> PDQFRAIIESPEGAGHVGYQYRRNTGSTMRMVSDVLDERVSLWDFHCDPSGNVIQPGPNVDSRQYLQAAIDYVSSNGGGTITIPAGYTWYLGSYGVGGIAGHSGIIQLRSNVNLNIEGRIHLSPFFDLKPFQVFVGFDNGDPASSGNLENCHIYGHGVVDFGGYEFGASSQLRNGVAFGRSYNCSVTGITFQNGDVTWAITLGWNGYGSNCYVRKCRFINLVNSSVNANHSTVYVNCPYSGVESCYFSMSSSFARNIACSVALHQHDTFYRGSTVNGYCRGAYVVMHAAEAAGAGSYAYNMQVENNIAVIYGQFVILGSDVTATVSGHLNDVIVSGNIVSIGERAAFSAPFGAFIDIGPDNSGASNVQDIQRVLVTGNSFYAPANITDSAAITLRANLNGCTFIANNFDCRYMVYNAPGTTSPVVQNLVWDKSNVIGGTHANQRAGQNLFDMQFASVVNSTIEVQLSCEDLSMFSCILFPASCQLSYSKITVDSAWTKSMSNTAVFEGNQQAGANVYVSYPATVNLTSYNTQGAVPFFSTDTNYAWVTSAYSLSINENLDFSPPATYTNKANGQLVGVGYNEIGGVRSVSVRLML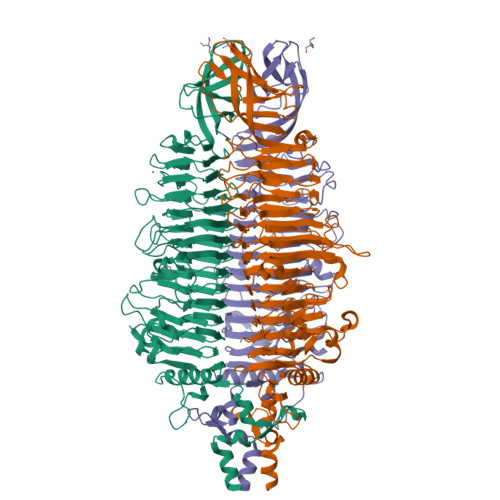QRQV>SVTTIPFWHSMEGELGKEVDSLAQRFNAENPDYKIVPTYKGNYEQNLSAGIAAFRTGNAPAILQVYEVGTATMMASKAIKPVYDVFKEAGIQFDESQFVPTVSGYYSDSKTGHLLSQPFNSSTPVLYYNKDAFKKAGLDPEQPPKTWQDLADYAAKLKASGMKCGYASGSQGSIQLENFSAWNGLPFASKNNGFDGTDAVLEFNKPEQVKHIAMLEEMNKKGDFSYVGRKDESTEKFYNGDCAMTTASSGSLANIREYAKFNYGVGMMPYDADAKDAPQNAIIGGASLW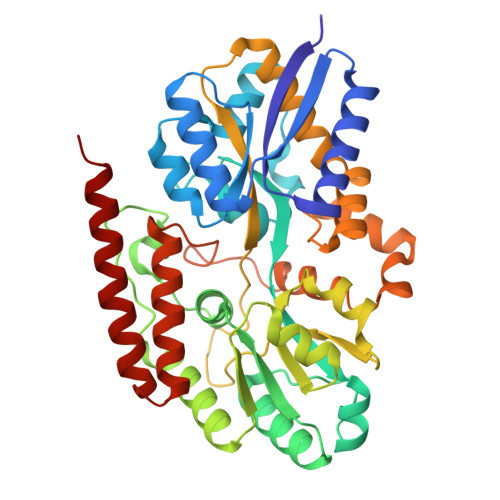VMQGKDKETYTGVAKFLDFLAKPENAAEWHQKTGYLPITKAAYDLTREQGFYEKNPGADTATRQMLNKPPLPFTKGLRLGNMPQIRVIVDEELESVWTGKKTPQQALDTAVERGNQLLRRFEKSTKS[2x]>[2x]GSHMSTNKITFLLNWEAA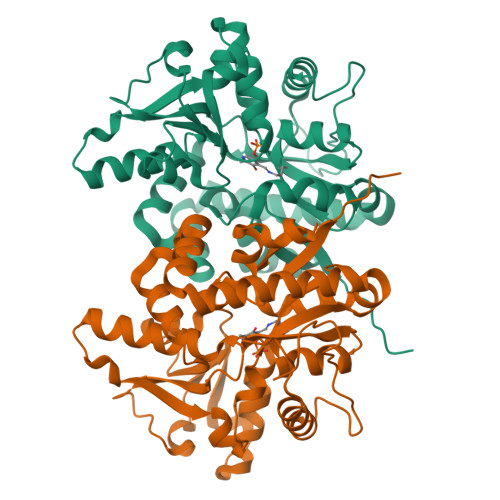PYHIPVYLANIKGYFKDENLDIAILEPSNPSDVTELVGSGKVDMGLKAMVHTLAAKARGFPVTSIGSLLDEPFTGICYLEGSGITSDFQSLKGKRIGYVGEFGKIQVDELTKHYGMTPDDYVAVRCGMNVAKYILEGTIDCGIGIECIQQVELEEALKEQGKDSNDAKMLRIDKLAELGCCCFCTILYIANDKFIAENPQAVKKFLKAIKRATDYMLAHPREAWAEYGNFKPTMQTDLNTKKFQRCYAYFSESLYNVHRDWRKVNNYGKRLDILPENYVPNYTNEYLSWPEPKEVDDPEKAQDLMLKHQEECKTCGGYKRLVLA>[2x]VQGPPSPGYYPSSQITSLGFDQGYTNLWGPQHQRVDQGSLTIWLDSTSGSGFKSINRYRSGYFGANIKLQSGY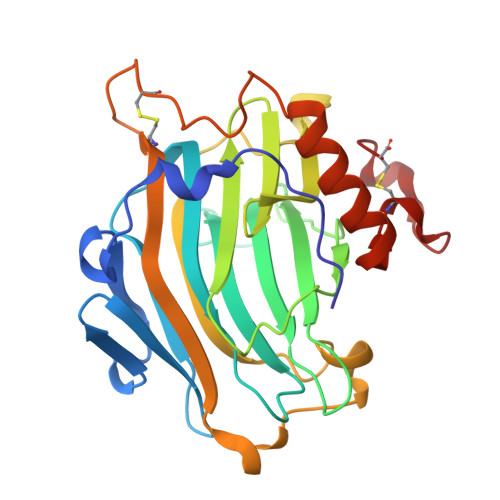TAGVITSFYLSNNQDYPGKHDEIDIEFLGTIPGKPYTLQTNVFIEGSGDREMRIHLWFDPTQDYHNYAIYWTPSEIIFFVDDVPIRRYPRKSDATFPLRPLWVYGSVWDASSWATENGKYKADYRYQPFVGKYEDFKLGSCTVEAASSCNPASVSPYGQLSQQQVAAMEWVQKNYMVYNYCDDPTRDHTLTPEC> MKIFSKCELARKLKSMGMDGFHGYSLANWVCMAEYESNFNTQAFNGRNSNGSSDYGIFQLNSKWWCKSNSHSSANACNIMCSKFLDDNIDDDIAC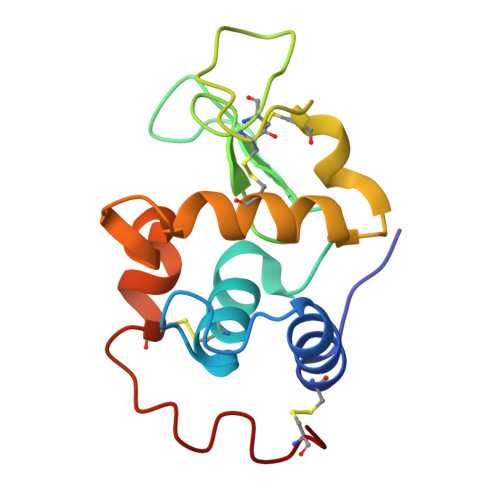AKRVVKDPNGMSAWVAWVKHCKGKDLSKYLASCNL> D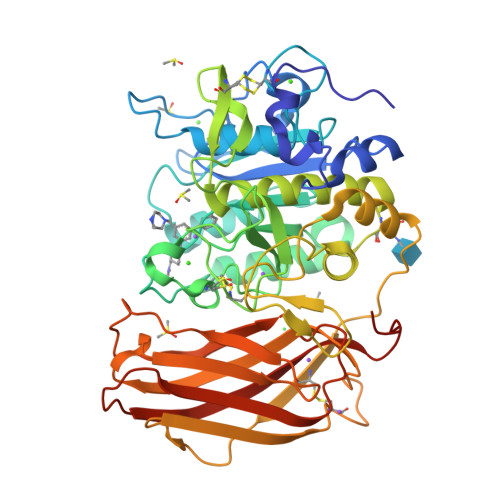VYQEPTDPKFPQQWYLSGVTQRDLNVKAAWAQGYTGHGIVVSILDDGIEKNHPDLAGNYDPGASFDVNDQDPDPQPRYTQMNDNRHGTRCAGEVAAVANNGVCGVGVAYNARIGGVRMLDGEVTDAVEARSLGLNPNHIHIYSASWGPEDDGKTVDGPARLAEEAFFRGVSQGRGGLGSIFVWASGNGGREHDSCNCDGYTNSIYTLSISSATQFGNVPWYSEACSSTLATTYSSGNQNEKQIVTTDLRQKCTESHTGTSASAPLAAGIIALTLEANKNLTWRDMQHLVVQTSKPAHLNANDWATNGVGRKVSHSYGYGLLDAGAMVALAQNWTTVAPQRKCIIDILTEPKDIGKRLEVRKTVTACLGEPNHITRLEHAQARLTLSYNRRGDLAIHLVSPMGTRSTLLAARPHDYSADGFNDWAFMTTHSWDEDPSGEWVLEIENTSEANNYGTLTKFTLVLYGTASGSLVPRGSHHHHHH ethyl 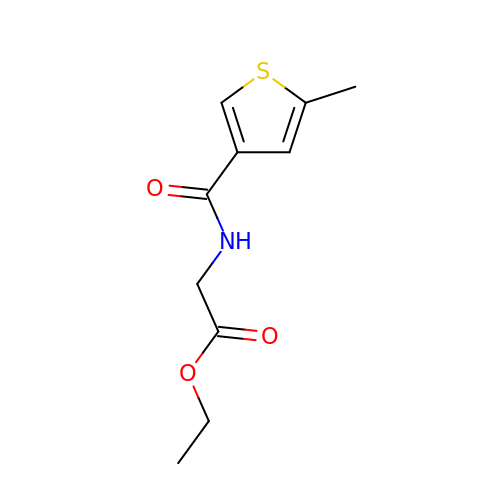N-[(5-methylthiophen-3-yl)carbonyl]glycinate | C10 H13 N O3 S | PMDIXZXNNWYFNT-UHFFFAOYSA-N> GMDYQEYQQFLARINTARDACVAKDIDVDLLMARHDYFGRELCKSLNIEYRNDVPFIDIILDIRPEVDPLTIDAPHITPDNYLYINNVLYIIDYKVSVSNESSVITYDKYYELTRDISDRLSIPIEIVIIRIDPVSRDLHINSDRFKELYPTIVVDINFNQFFDLKQLLYEKFGDDEEFLLKVAHGDFTLTAPWCKTGCPEFWKHPIYKEFKMSMPVPERRLFEESVKFNAYESERWNTNLVKIREYTKKDYSEHISKSAKNIFLASGFYKQPNKNEISEGWTLMVERVQDQREISKSLHDQKPSIHFIWGAHNPGNSNNATFKLILLSKSLQSIKGISTYTEAFKSLGKMMDIGDKAIEYEEFCMSLKSKARSSWKQIMNKKLEPKQINNALVLWEQQFMINNDLIDKSEKLKLFKNFCGIGKHKQFKNKMLEDLEVSKPKILDFDDANMYLASLTMMEQSKKILSKSNGLKPDNFILNEFGSRIKDANKETYDNMHKIFETGYWQCISDFSTLMKNILSVSQYNRHNTFRIAMCANNNVFAIVFPSADIKTKKATVVYSIIVLHKEEENIFNPGCLHGTFKCMNGYISISRAIRLDKERCQRIVSSPGLFLTTCLLFKHDNPTLVMSDIMNFSIYTSLSITKSVLSLTEPARYMIMNSLAISSNVKDYIAEKFSPYTKTLFSVYMTRLIKNACFDAYDQRQRVQLRDIYLSDYDITQKGIKDNRELTSIWFPGSVTLKEYLTQIYLPFYFNAKGLHEKHHVMVDLAKTILEIECEQRENIKEIWSTNCTKQTVNLKILIHSLCKNLLADTSRHNHLRNRIENRNNFRRSITTISTFTSSKSCLKIGDFRKEKELQSVKQKKILEVQSRKMRLANPMFVTDEQVCLEVGHCNYEMLRNAMPNYTDYISTKVFDRLYELLDKKVLTDKPVIEQIMDMMIDHKKFYFTFFNKGQKTSKDREIFVGEYEAKMCMYAVERIAKERCKLNPDEMISEPGDGKLKVLEQKSEQEIRFLVETTRQKNREIDEAIEALATEGYESNLGKIEKLSLGKAKGLKMEINADMSKWSAQDVFYKYFWLIALDPILYPQEKERILYFMCNYMDKELILPDELLFNLLDQKVAYQNDIIATMTNQLNSNTVLIKRNWLQGNFNYTSSYVHSCAMSVYKEILKEAITLLDGSILVNSLVHSDDNQTSITIVQDKMENDKIIDFAMKEFERACLTFGCQANMKKTYVTNCIKEFVSLFNLYGEPFSIYGRFLLTSVGDCAYIGPYEDLASRISSAQTAIKHGC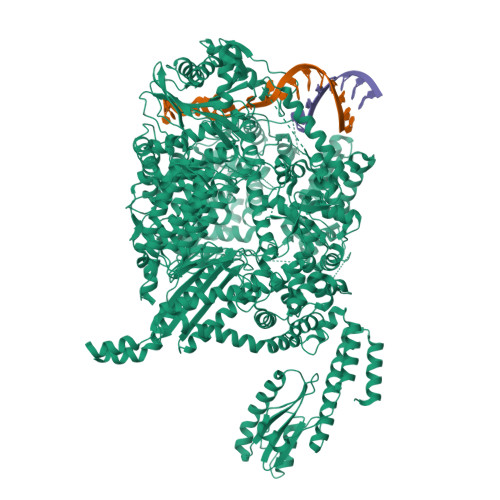PPSLAWVSIAISHWMTSLTYNMLPGQSNDPIDYFPAENRKDIPIELNGVLDAPLSMISTVGLESGNLYFLIKLLSKYTPVMQKRESVVNQIAEVKNWKVEDLTDNEIFRLKILRYLVLDAEMDPSDIMGETSDMRGRSILTPRKFTTAGSLRKLYSFSKYQDRLSSPGGMVELFTYLLEKPELLVTKGEDMKDYMESVIFRYNSKRFKESLSIQNPAQLFIEQILFSHKPVIDFSGIRDKYINLHDSRALEKEPDILGKVTFTEAYRLLMRDLSSLELTNDDIQVIYSYIILNDPMMITIANTHILSIYGSPQRRMGMSCSTMPEFRNLKLIHHSPALVLRAYSKNNPDIQGADPTEMARDLVHLKEFVENTNLEEKMKVRIAMNEAEKGQRDIVFELKEMTRFYQVCYEYVKSTEHKIKVFILPAKSYTTTDFCSLMQGNLIKDKEWYTVHYLKQILSGGHKAIMQHNATSEQNIAFECFKLITHFADSFIDSLSRSAFLQLIIDEFSYKDVKVSKLYDIIKNGYNRTDFIPLLFRTGDLRQADLDKYDAMKSHERVTWNDWQTSRHLDMGSINLTITGYNRSITIIGEDNKLTYAELCLTRKTPENITISGRKLLGSRHGLKFENMSKIQTYPGNYYITYRKKDRHQFVYQIHSHESITRRNEEHMAIRTRIYNEITPVCVVNVAEVDGDQRILIRSLDYLNNDIFSLSRIKVGLDEFATIKKAHFSKMVSFEGPPIKTGLLDLTELMKSQDLLNLNYDNIRNSNLISFSKLICCEGSDNINDGLEFLSDDPMNFTEGEAIHSTPIFNIYYSKRGERHMTYRNAIKLLIERETKIFEEAFTFSENGFISPENLGCLEAVVSLIKLLKTNEWSTVIDKCIHICLIKNGMDHMYHSFDVPKCFMGNPITRDINWVMFREFINSLPGTDIPPWNVMTENFKKKCIALINSKFETQRDFSEFTKLMKKEGGRSNIEFD> KAHVLAASVEQATENFLEKGDKIAKESQFLKEELVVAVEDVRKQGDLMKSAAGEFADDPCSSVKRGNMVRAARALLSAVTRLLILADMADVYKLLVQLKVVEDGILKLRNAGN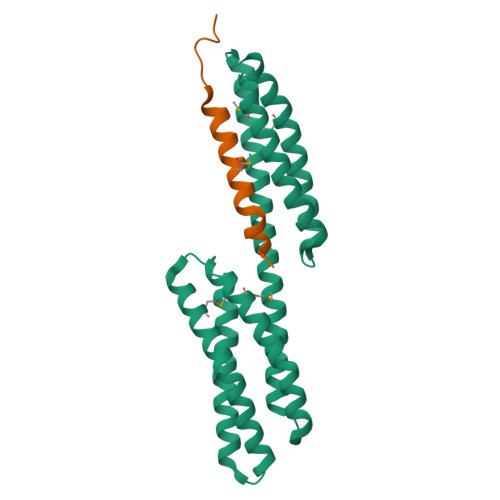EQDLGIQYKALKPEVDKLNIMAAKRQQELKDVGNRDQMAAARGILQKNVPILYTASQACLQHPDVAAYKANRDLIYKQLQQAVTGISNAAQA;> HPTNVQRLAEPSQMLKHAVVNLINYQDDAELA3-[(1E,7E)-8-(2,6-dioxo-1,2,3,6-tetrahydropyrimidin-4-yl)-3,6-dioxa-2,7-diazaocta-1,7-dien-1-yl]benzoic acid | C15 H14 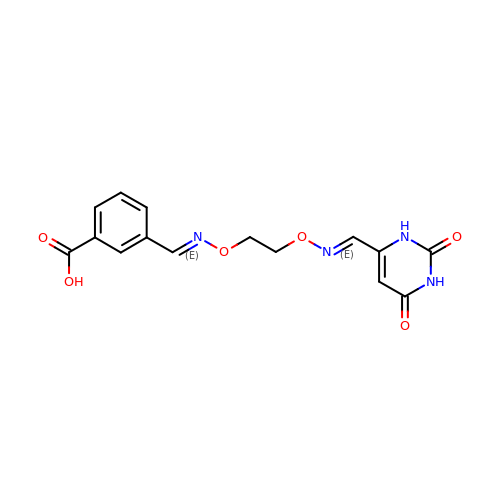N4 O6 | TUYDQQMKXSQIQG-GONBZBRSSA-N> SWESHKSGRE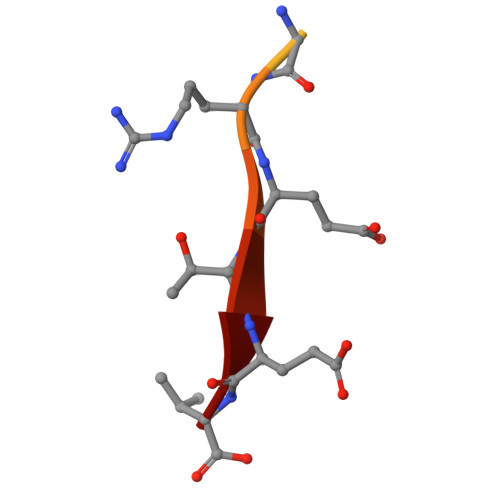TEV> S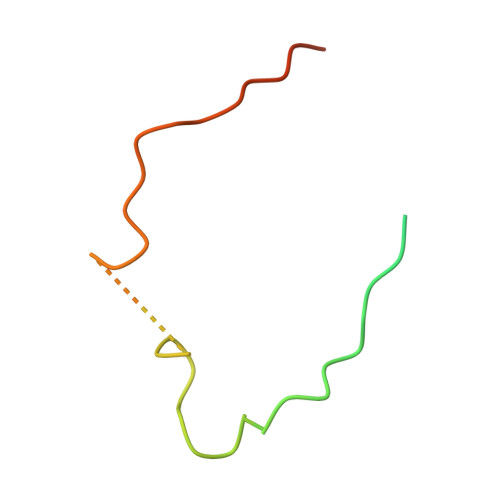NGQESPTAENARLLAQKRGALQGSAWQVSSEDVRWDTFPLGRMPGQTEDPAELMLENYDTMYLLDQPVLE>[60x]MGSSHHHHHHSQDPKNIKIMRLVTGEDIIGNISESQGLITIKKAFVIIPMQATPGKPVQLVLSPWQPYTDDKEIVIDDSKVITITSPK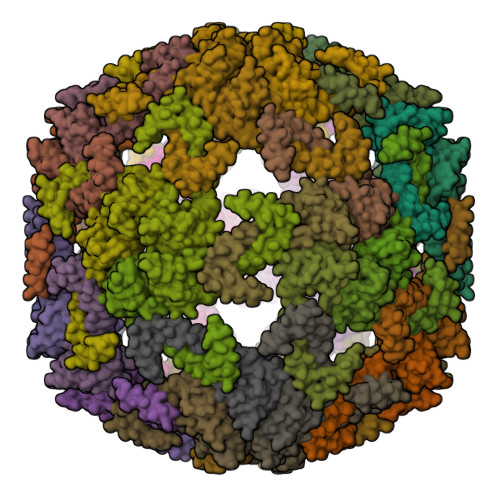DDIIKSYESHTRVLENKQVEEILRLEKEIEDLQRMKEQQELSLTEASLQKLQERRDQELRRLEEE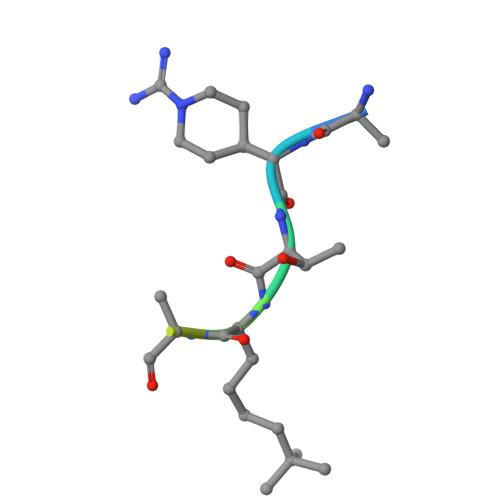> ARTXQTARKS> PDVVLVNGGEPPNPLIPTGTNDSNGGRIIDRLFAGLMSYDAVGKPSLEVAQSIESADNVNYRITVKPGWKFTDGSPVTAHSFVDAWNYGALSTNAQLQQHFFSPIEGFDDVAGAPGDKSRTTMSGLRVVNDLEFTVRLKAPTIDFTLALGHSSFYPLPDSAFRDMAAFGRNPIGNGPYKLADGPAGPAWEHNVRIDLV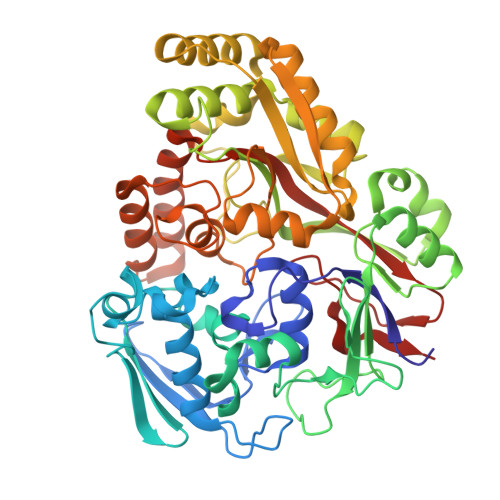PNPDYHGNRKPRNKGLRFEFYANLDTAYADLLSGNLDVLDTIPPSALTVYQRDLGDHATSGPAAINQTLDTPLRLPHFGGEEGRLRRLALSAAINRPQICQQIFAGTRSPARDFTARSLPGFDPNLPGNEVLDYDPQRARRLWAQADAISPWSGRYAIAYNADAGHRDWVDAVANSIKNVLGIDAVAAPQPTFAGFRTQITNRAIDSAFRAGWRGDYPSMIEFLAPLFTAGAGSNDVGYINPEFDAALAAAEAAPTLTESHELVNDAQRILFHDMPVVPLWDYISVVGWSSQVSNVTVTWNGLPDYENIVKA> MRGSHHHHHHGSHDLPCLNLEPPKMLKLSPLLRALQDRGPIHRVRTPAGDEAWLVTRHAELKQLLHDERIGRTHPDPPSAAQYVRSPFLDLLISDADA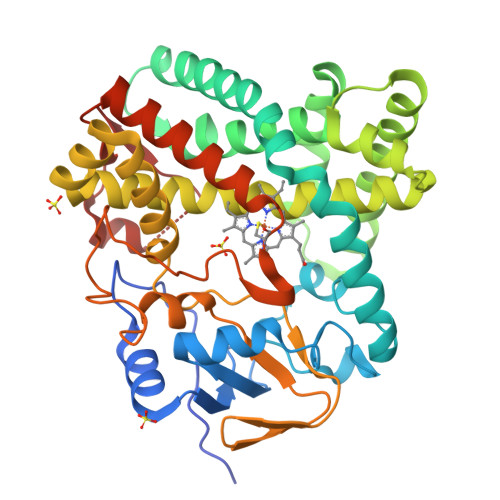ESGRRQHAETRRLLTPLFSARRVLEMQPKVEEAADTLLDAFIAQGPPGDLHGELTVPFALTVLCEVIGVPPQRRAELTTLLAGIAKLDDREGAVRAQDDLFGYVAGLVEHKRAEPGPDIISRLNDGELTEDRVAHLAMGLLFAGLDSVASIMDNGVVLLAAHPDQRAAALADPDVMARAVEEVLRTARAGGSVLPPRYASEDMEFGGVTIRAGDLVLFDLGLPNFDERAFTGPEEFDAARTPNPHLTFGHGIWHCIGAPLARLELRTMFTKLFTRLPELRPELPVEQLRLKEGQLSGGFAELRVVW(6~{S},9~{a}~{S})-6-[(2~{S})-butan-2-yl]-8-[(4-methoxynaphthalen-1-yl)methyl]-4,7-bis(oxidanylidene)-~{N}-[4,4,4-tris(fluoranyl)butyl]-3,6,9,9~{a}-tetrahydro-2~{H}-pyrazino[1,2-a]pyrimidine-1-carboxamide 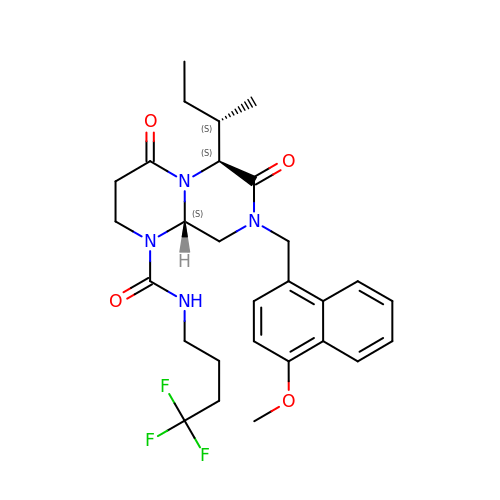| C28 H35 F3 N4 O4 | ZCPTWZWAPHZUMM-UODBTFMRSA-N>[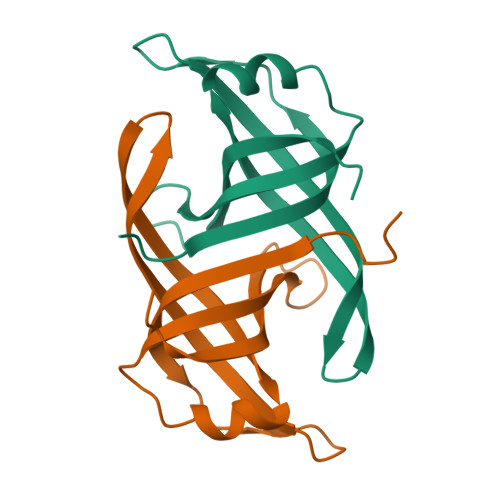2x]GSHMGFTNLVSLAALIEKAFPIRYTPAGIPVLDIILKHESWQEENGQQCLVQLEIPARILGRQAEEWQYRQGDCATVEGFLAQKSRRSLMPMLRIQNIKEYKG> SGVFQLQLQEFINERGVLASGRPCEPGCRTFFRVCLKHFQAVVSP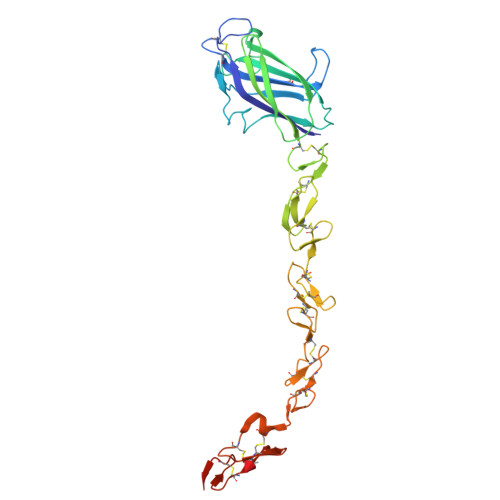GPCTFGTVSTPVLGTNSFAVRDDSSGGGRNPLQLPFNFTWPGTFSLIIEAWHAPGDDLRPEALPPDALISKIAIQGSLAVGQNWLLDEQTSTLTRLRYSYRVICSDNYYGDNCSRLCKKRNDHFGHYVCQPDGNLSCLPGWTGEYCQQPICLSGCHEQNGYCSKPAECLCRPGWQGRLCNECIPHNGCRHGTCSTPWQCTCDEGWGGLFCDQDLNYCTHHSPCKNGATCSNSGQRSYTCTCRPGYTGVDCELELGSHHHHHHHH>MTKGKKLVWEEHFNGKELDTKNWNFELGDGCPNCGWGNSERQLYTKTNHKMENGKLVITAKKEGTQYTSTRITTQGKKEFQYGYIEARAKLPVGKGIWPAFWMLGSNIKTVGWPQCGEIDILEYVGKEPHMVFTS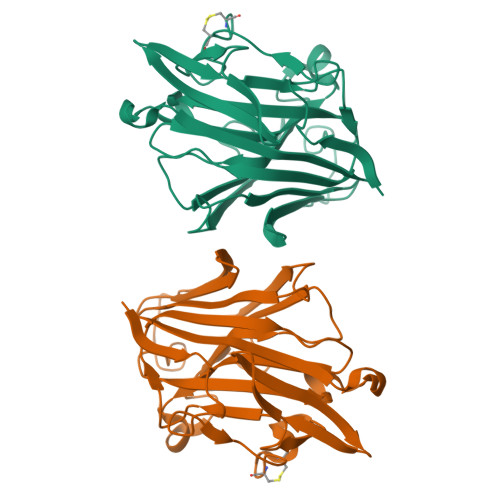LHTTASHGNTINTKRTRIDTIEQGFHLYAIDWTKDKMDFFVDNILVYTFNPTDKTEAIWPYDQPFYFIINMAIGGNFGGPEVDDAIFPQDFSIDYIKVYQ[2x]>[6x]TQSPALIASQSLGRCTQAKDREGWLALMADDVVIETPIGKSVTNPDGSGIKGKEAVGAFWDTHIADDRVTVTCEETFPSSSPDEIAHILVA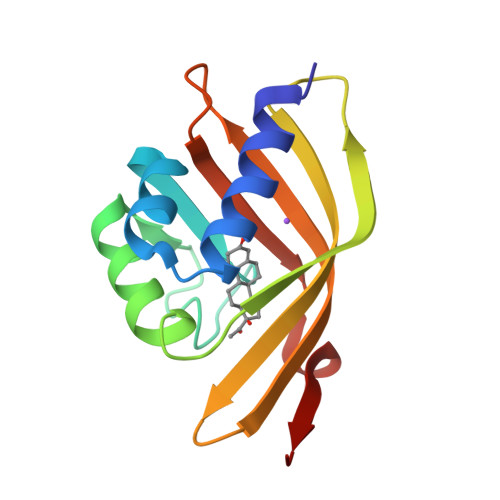HAEFDGGFTSEVRGVFTYRVNKAGLITNLRGYYNLDMMTFGNQ> SEFENPLKRLLVPGEEWEFEVTAFYRGRQVFQQTISCPEGLRLVGSEVGDRTLPGWPVTLPDPGMSLTDRGVMSYVRHVLSCLGGGLALWRAGQWLWAQRLGHCHTYWAVSEELLPNSGHGPDGEVPKDKEGGVFDLGPFIVDLITFTEGSGRSPRYALWFCVGESWPQDQPWTKRLVMVKVVPTCLRALVEMARVGGASSLENTVDLHISNSHPLSLTSDQYKAYLQDLVE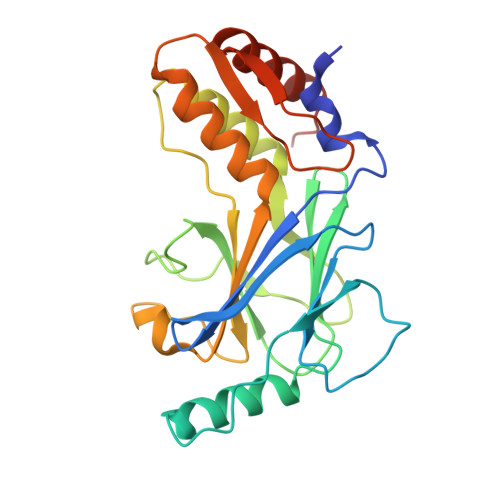GMDFQGPGES> GAMADTCMSRIVKEYKVI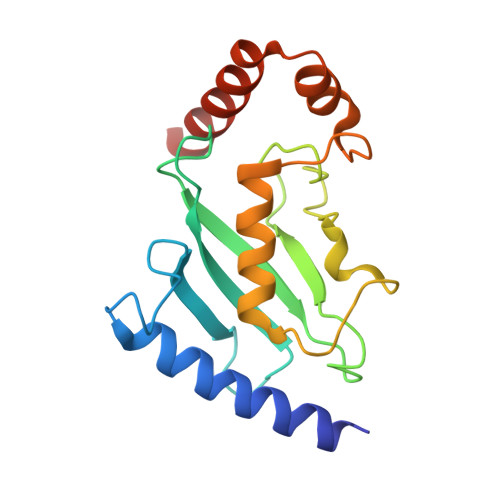LKTLASDDPIANPYRGIIESLNPIDETDLSKWEAIISGPSDTPYENHQFRILIEVPSSYPMNPPKISFMQNNILHCNVKSATGEICLNILKPEEWTPVWDLLHCVHAVWRLLREPVCDSPLDVDIGAIIRCGDMSAYQGIVKYFLAERERINNH>[6x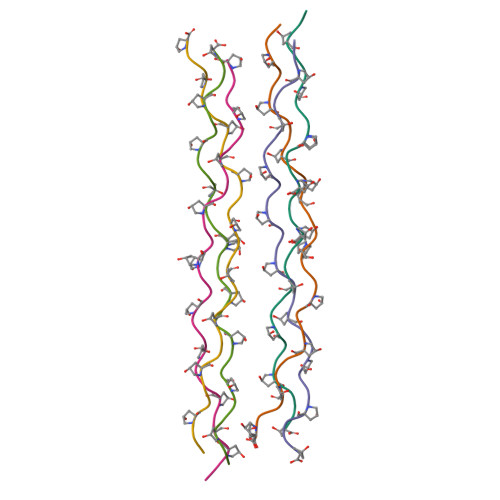]GPPGPPGPPGPPALPGPPGPPGPPGPP>[8x]AGSMKLLNIKINEFAVTANTEAGDELYLQLPHTPDSQHSINHEPLDDDDFVKEVQEIC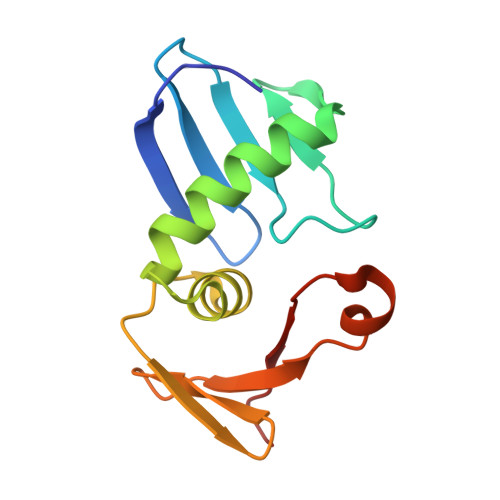DEYFGKGDRTMARLSYAGGQAYDSYTEEDGVYTTNTGDQFVEHSYADYYNVEVYCKADLV The Nef protein is an accessory gene product of HIV and SIV that is dispensable for virus spread in experimental ex vivo cell culture systems. Thus, Nef is an important factor for AIDS pathogenesis. To achieve this multitude of activities, Nef has evolved as versatile adaptor for protein interactions that lacks intrinsic enzymatic activity, which allows the viral protein to affect a wide range of host cell protein sorting and signal transduction processes. We thus chose a strategy aimed at wrapping the surface of Nef by the combination of different, physically linked, target domains and the iterative optimization of domain composition and linker segments.

Attachment of the cytoplasmic domain of CD4, however, which is the smallest unit tested, turned out to be suitable for in vitro characterization and amenable for structure-function based binding improvements. In this study we engineered a 10.0 kDa protein (86 amino acids) that binds to HIV-1 Nef in the low nano-molar range. Indeed, we show here that the binding affinity of a designed protein inhibitor to HIV-1 Nef is increased from 250 to 26 nM by fusion of two structural elements and further lead optimization. This fusion protein is the tightest binder to Nef known to date and supposedly covers a large surface on the target protein. Thus, a protein construct was designed that simultaneously covered three interaction sites of Nef, wrapping its functional surface sites to render the protein non-functional. Unfortunately, there was no electron density visible that would unambiguously account for the CD4 part of the inhibitory molecule. However, the resolution achieved was sufficient to show that the N-terminal chain of Nef in one complex of the asymmetric unit was bended away such that the binding site distal to the PxxP motif on face the F94–W117 gatekeeper residues could become accessible for other interactions. However, NMR spectroscopic analysis strongly support the displacement of the before mentioned newly identified N-terminal helix by the CD4 segment. Mutagenesis analyses showed that the CD4 dileucine motif is required for binding to Nef, while a C-terminal cysteine-rich motif, which was shown to form an intermolecular zinc-finger with the unique domain of Hck, did not contribute to the interaction.

>[2x]GAMASSNTAATNADSAWLEAQEEEEVGFPVRPQVPLRPMTYKAALDISHFLKEKGGLEGLIWSQRRQEILDLWIYHTQGYFPDWQNYTPGPGIRYPLTFGWCFKLVPVEPEKVEEANEGENNSLLHPMSLHGMEDAEKEVLVWRFDSKLAFHHMARELHPEYYKDA;>[2x]MEDIIVVALYDYVSWSPDDLSFQKGDQMVVLEESGEWWKARSLATRKEGYIPSNYVARVDSGGGTSGGGRHRRRQAERMSQIKRLLSEKK>GSHMSTITRPIIELSNTADKIAEGNLEAEVPHQNRADEIGILAKSIERLRRSLKQLADDGTLLMAGVSHDLRTPLTRIRLATEMMSEQDGYLAE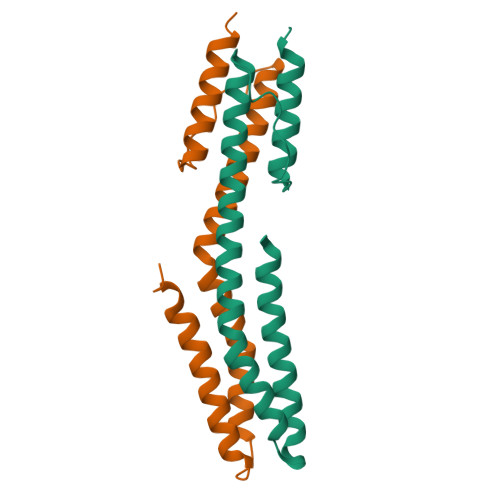SINKDIEECNAIIEQFIDYL[2x]> MTTYLEFIQQNEERDGVRFSWNVWPSSRLEATRMVVPVAALFTPLKERPDLPPIQYEPVLCSRTTCRAVLNPLCQVDYRAKLWACNFCYQRNQFPPSYAGISELNQPAELLPQFSSIEYVVLRGPQMPLIFLYVVDTCMEDEDLQALKESMQMSLSLLPPTALVGLITFGRMVQVHELGCEGISKSYVFRGTKDLSAKQLQEMLGLSKVPLTQATRGPQVQQPPPSNRFLQPVQKIDMNLTDLLGELQRDPWPVPQGKRPLRSSG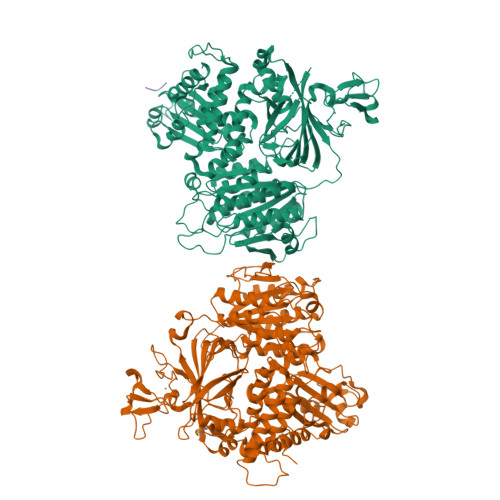VALSIAVGLLECTFPNTGARIMMFIGGPATQGPGMVVGDELKTPIRSWHDIDKDNAKYVKKGTKHFEALANRAATTGHVIDIYACALDQTGLLEMKCCPNLTGGYMVMGDSFNTSLFKQTFQRVFTKDMHGQFKMGFGGTLEIKTSREIKISGAIGPCVSLNSKGPCVSENEIGTGGTCQWKICGLSPTTTLAIYFEVVNQHNAPIPQGGRGAIQFVTQYQHSSGQRRIRVTTIARNWADAQTQIQNIAASFDQEAAAILMARLAIYRAETEEGPDVLRWLDRQLIRLCQKFGEYHKDDPSSFRFSETFSLYPQFMFHLRRSSFLQVFNNSPDESSYYRHHFMRQDLTQSLIMIQPILYAYSFSGPPEPVLLDSSSILADRILLMDTFFQILIYHGETIAQWRKSGYQDMPEYENFRHLLQAPVDDAQEILHSRFPMPRYIDTEHGGSQARFLLSKVNPSQTHNNMYAWGQESGAPILTDDVSLQVFMDHLKKLAVSSAA;> AMGSPIQVIENDRASRGGQVYATNTRGQIPPLVTTDCMIQDQGNASPRFIRCTTYCFPCTSDMAKQAQIPLAAVIKPFATIPSNESPLYLVNHGESGPVRCNRCKAYMCPFMQFIEGGRRYQCGFCNCVNDVPPFYFQHLDHIGRRLDHYEKPELSLGSYEYVATLDYCRKSKPPNPPAFIFMIDVSYSNIKNGLVKLICEELKTMLEKIPKEEQEETSAIRVGFITYNKVLHFFNVKSNLAQPQMMVVTDVGEVFVPLLDGFLVNYQESQSVIHNLLDQIPDMFADSNENETVFAPVIQAGMEALKAADCPGKLFIFHSSLPTAEAPGKLKNRDDKKLVNTDKEKILFQPQTNVYDSLAKDCVAHGCSVTLFLFPSQYVDVASLGLVPQLTGGTLYKYNNFQMHLDRQQFLNDLRNDIEKKIGFDAIMRVRTSTGFRATDFFGGILMNNTTDVEMAAIDCDKAVTVEFKHDDKLSEDSGALIQCAVLYTTISGQRRLRIHNLGLNCSSQLADLYKSCETDALINFFAKSAFKAVLHQPLKVIREILVNQTAHMLACYRKNCASPSAASQLILPDSMKVLPVYMNCLLKNCVLLSRPEISTDERAYQRQLVMTMGVADSQLFFYPQLLPIHTLDVKSTMLPAAVRCSESRLSEEGIFLLANGLHMFLWLGVSSPPELIQGIFNVPSFAHINTDMTLLPEVGNPYSQQLRMIMGIIQQKRPYSMKLTIVKQREQPEMVFRQFLVEDKGLYGGSSYVDFLCCVHKEICQLLN;> LPPPFGPGM>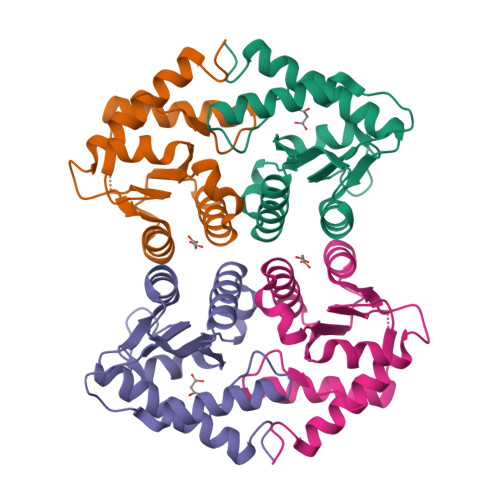[2x]MTLEEVRGQDTVPESTARMQGAGKALHELLLSAQRQGCLTAGVYESAKVLNVDPDNVAFCVLAAGEEDEGDIALQIHFTLIQAFCCENDIDIVRVGDVQRLAAIVGAGEEAGAPGDLHCILISNPNEDAWKDPALEKLSLFCEESRSVNDWVPSITLPE Kainate receptors, a subclass of ionotropic glutamate receptors, are tetrameric ligand-gated ion channels that mediate excitatory neurotransmission. Each KAR subunit has a multi-domain organization, including the amino-terminal domain (ATD), involved in receptor assembly and trafficking, the ligand-binding domain (LBD) that binds agonists, competitive antagonists and positive allosteric modulators (PAMs), the transmembrane domain (TMD), which forms an ion-conducting channel, and the carboxy-terminal domain, which determines surface expression, synaptic localization and interactions with intracellular proteins. Here we present cryo-electron microscopy structures of the kainate receptor GluK2 in the presence of the agonist glutamate and the positive allosteric modulators lectin concanavalin A and BPAM344. Concanavalin A and BPAM344 inhibit kainate receptor desensitization and prolong activation by acting as a spacer between the amino-terminal and ligand-binding domains and a stabilizer of the ligand-binding domain dimer interface, respectively.

The ConA-bound group of GluK2 particles includes two subgroups, with one or two ConA dimers bound. One protomer in the ConA dimer contacts the ATD, whereas the second interacts with the LBD. There were two types of ConA–LBD contacts, with the predominant type I contacts involving the A or C subunit LBD and type II contact involving the B or D subunit LBD. The type I ConA–LBD contact is mediated by carbohydrates attached to N546, the glycosylation site conserved among GluK1–3 subunits, and the type II contact appears to also involve carbohydrates attached to N751, the glycosylation site conserved over all GluK subunits. Although single N546Q and N751Q substitutions substantially reduced the steady-state currents, dramatic current reduction was only achieved in the double mutant N546Q/N751Q, suggesting the interchangeable capability of carbohydrates attached to N546 and N751 to serve as ConA contact points. Our experiments with mutant GluK2 channels therefore confirmed glycosylation of residues N378, N546 and N751 to be critical for PAM action of lectin ConA on GluK2 receptors.

>[2x]ADTIVAVELDTYPNTDIGDPSYPHIGIDIKSVRSKKTAKWNMQNGKVGTAHIIYNSVDKRLSAVVSYPNADSATVSYDVDLDNVLPEWVRVGLSASTGLYKETNTILSWSFTSKLKSNSTHETNALHFMFNQFSKDQKDLILQGDATTGTDGNLELTRVSSNGSPQGSSVGRALFYAPVHIWESSAVVASFEATFTFLIKSPDSHPADGIAFFISNIDSSIPSGSTGRLLGLFPDAN>MGFSDLRDKVVIVTGASMGIGRAIAERFVDEGSKVIDLSIHDPGEAKYDHIECDVTNPDQVKASIDHIFKEYGSISVLVNNAGIESYGKIESMSMGEWRRIIDVNLFGYYYASKFAIPYMIRSRDPSIVNISSVQASIITKNASAYVTSKHAVIGLTKSIALDYAPLLRCNAVCPATIDTPLVRKAAELEVGSDPMRIEKKISEWGHEH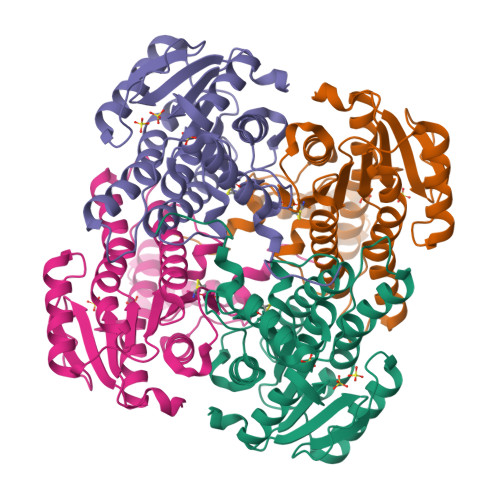PMQRIGKPQEVASAVAFLASREASFITGTCLYVDGGLSIRAPISTPELEHHHHHH[2x]> DRVAQQANELIKRVASELEKNRKKLIKQEQELAD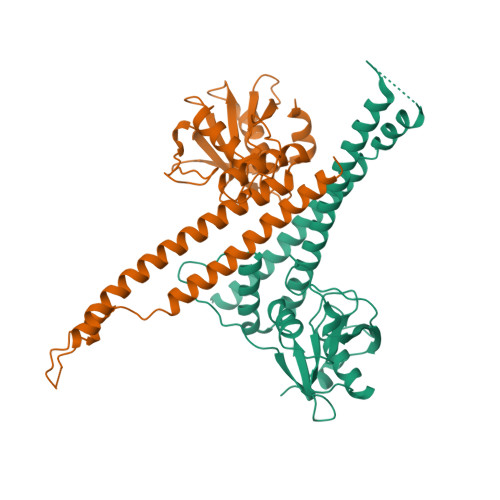TETAELVRQKGELLTTYVHQVPNDQSSVRLDNYYTGKELEIELDVALTPSQNAQRYFKKYQKLKEAVKHLTNLIEETKSTIVYLESVDTMLGQASLAEIDEIREELIETGYLKRRHREKIHKRQKPERYLATDGKTIILVGKNNLQNDELTFKMAKKGELWFHAKDIPGSHVVITDNLDPSDEVKTDAAELAAYFSKARHSNLVQVDMIEAKKLHKPTGGKPGFVTYRGQKTLRVTPTEDKIKSMKI;> RDRVAQQANELIKRVASELEKNRKKLIKQEQELADTETAELVRQKGEILTTYVHQVPNDQSSVRLDNYYTGKELEIELDVALTPSQNAQRYFKKYQKLKEAVKHLTNLIEETKSTIVYLESVDTMLGQASLAEIDEIREELIETGYLKRRHREKIHKRQKPERYLATDGKTIILVGKNNLQNDELTFKMAKKGELWFHAKDIPGSHVVITDNLDPSDEVKTDAAELAAYFSKARHSNLVQVDMIEAKKLHKPTGGKPGFVTYRGQKTLRVTPTEDKIKSMKI>MPTIDFTFCEINPKKGFGGANGNKISLFYNNELYMVKFPPKPSTHKEMSYTNGCFSEYVACHIVNSLGLKVQETLLGTYKNKIVVACKDFTTHQYELVDFLSLKNTMIELEKSGKDTNLNDVLYAIDNQHFIEPKVLKCFFWDMFVADTLLGNFDRHNGNWGFLRASNSKEYQIAPIFDCGSCLYPQADDVVCQKVLSNIDELNARIYNFPQSILKDDNDKKINYYDFLTQTNNKDCLDALLRIYPRIDMNKIHSIIDNTPFMSEIHKEFLHTMLDERKSKIIDVAHTRAIELSLQHKQAHSNPYDNADDLDNSNEYTPTPK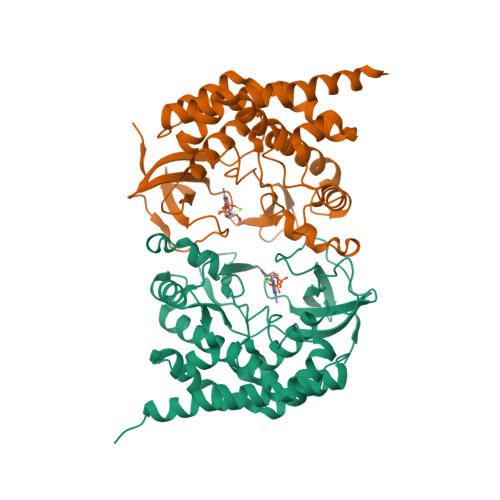RRR[4x]> MRSTQEERFEQRIAQETAIEPQDWMPDAYRKTLIRQIGQHAHSEIVGMLPQGNWITRAPTLRRKAILLAQVQDEAGHGLYLYSAAETLGCAREDIYQKMLDGRMKYSSIFNYPTLSWADIGVIGWLVDGAAIVNQVALCRTSYGPYARAMVKICKEESFHQRQGFEACMALAQGSEAQKQMLQDAINRFWWPALMMFGPNDDNSPNSARSLTWKIKRFTNDELRQRFVDNTVPQVEMLGMTVPDPDLHF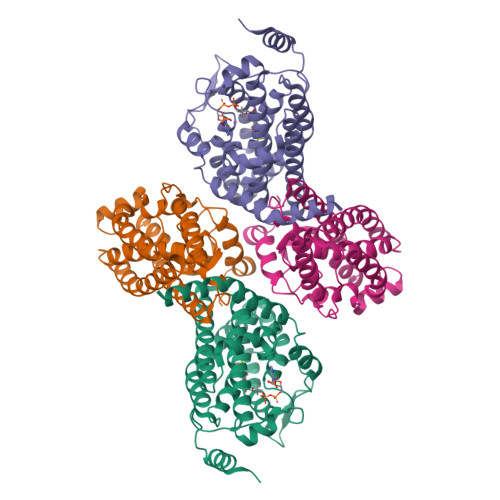DTESGHYRFGEIDWQEFNEVINGRGICNQERLDAKRKAWEEGTWVREAALAHAQKQHARKVA;>MGSSHHHHHHGSNQLTAYTLRLGDNCLVLSQRLGEWCGHAPELEIDLALANIGLDLLGQARNFLSYAAELAGEGDEDTLAFTRDERQFSNLLLVEQPNGNFADTIARQYFIDAWHVALFTRLMESRDPQLAAISAKAIKEARYHLRFSRGWLERLGNGTDVSGQKMQQAINKLWRFTAELFDADEIDIALSEEGIAVDPRTLRAAWEAEVFAGINEATLNVPQEQAYRTGGKKGLHTEHLGPMLAEMQYLQRVLPGQQW[2x]>HSWERLAVLVLLGAAACAAPPRGRILGGREAEAHARPYMASVQLNGAHLCGGVLVAEQWVLSAAHCLEDAADGKVQVLLGAHSLSQPEPSKRLYDVLRAVPHPDSQPDTIDHDLLLLQLSEKATLGPAVRPLPWQRVDRDVAPGTLCDVAGWGIVNHAGRRPDSLQHVLLPVLDRATCN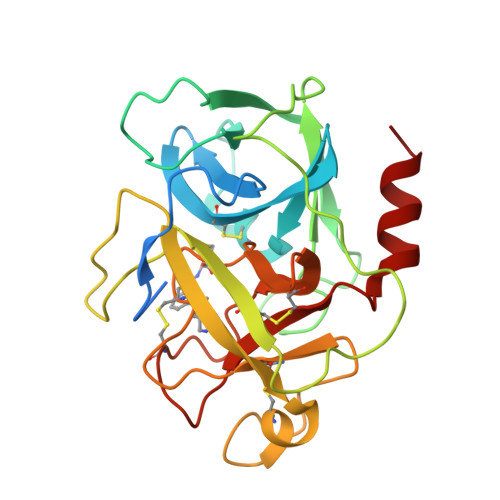RRTHHDGAITERLMCAESNRRDSCKGDSGGPLVCGGVLEGVVTSGSRVCGNRKKPGIYTRVASYAAWIDSVLASA[2x]>DERSWVYSPLHYSA[6x];>[6x]PVQLNLLYVQARDDILNGSHPVSFDKACEFAGFQCQIQFGPHNEQKHKAGFLDLKDFLPKEYVKQKGERKIFQAHKNCGQMSEIEAKVRYVKLARSLKTYGVS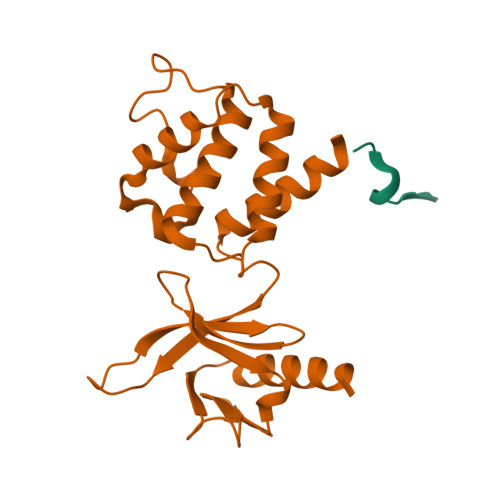FFLVKEKMKGKNKLVPRLLGITKECVMRVDEKTKEVIQEWSLTNIKRWAASPKSFTLDFGDYQDGYYSVQTTEGEQIAQLIAGYIDIILKKKKSKDHFG~{N}-[(2~{S})-1-[(3~{R},3~{a}~{R},6~{S},6~{a}~{S})-6-fluoranyl-3-oxidanyl-2,3,3~{a},5,6,6~{a}-hexahydrofuro[3,2-b]pyrrol-4-yl]-4-methyl-1-oxidanylidene-pentan-2-yl]-4-thiophen-2-yl-benzamide 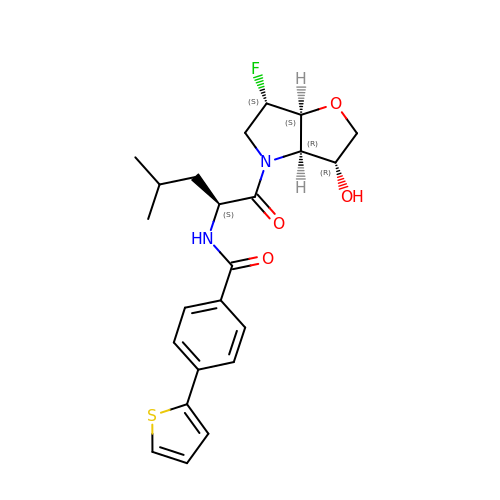| C23 H27 F N2 O4 S | PPPDNJKXIHLWJW-DSVUQQCSSA-N> MTREELLRENIELAKEHIEIMREILELLQKMEELLEKAR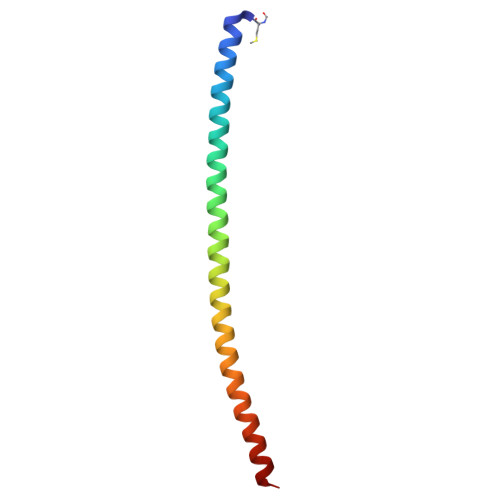GADEDVAKTIKELLRRLKEIIERNQRIAKEHEYIARERS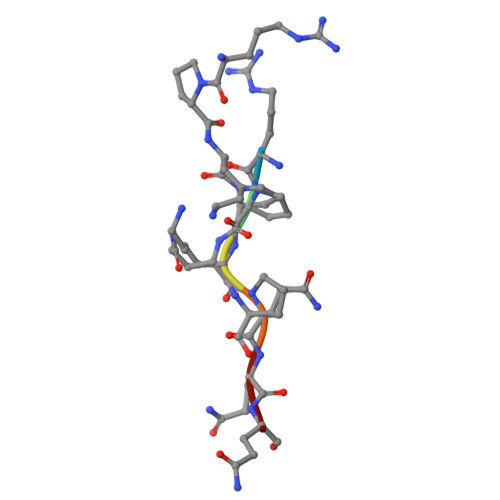> RPKPQQ>GPGSMSGPVTYTHDDAIGVIRMDDGKVNVLGPTMQQALNEAIDAADRDNVGALVIAGNHRVFSGGFDLKVLTSGEAKPAIDMLRGGFELSYRLLSYPKPVVIACTGHAIAMGAFLLCSGDHRVAAHAYNIQANEVAIGMTIPYAAMEVLKLRLTPSAYQQAAGLAKTFFGE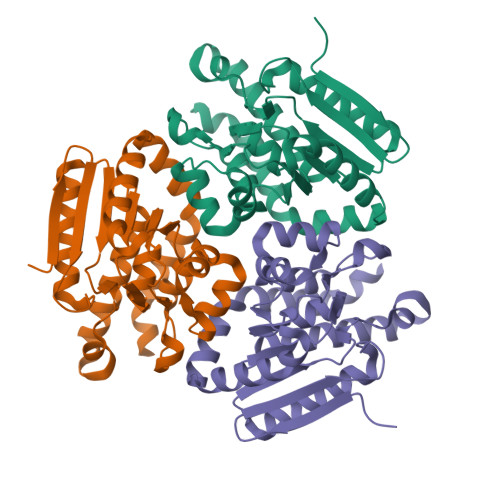TALAAGFIDEISLPEVVLSRAEEAAREFAGLNQQAHNATKLRARAEALKAIRAGIDGIEAEFGL[3x]>[2x]GSGHKSSPCDTNWRYYGDSCYGFFRHNLTWEESKQYCTDMNATLLKIDNRNIVEYIKARTHLIRWVGLSRQKSNE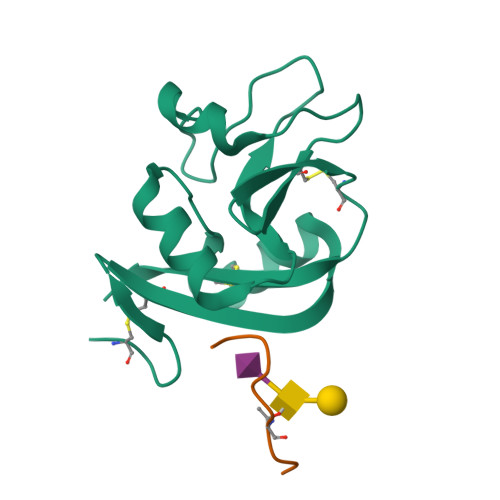VWKWEDGSVISENMFEFLEDGKGNMNCAYFHNGKMHPTFCENKHYLMCERKAG;>EGGVAMPGAEDDVVTPGC[2x]>[2x]IVGGRRARPHAWPFMVSLQLRGGHFCGATLIAPNFVMSAAHCVANVNVRAVRVVLGAHNLSRREPTRQVFAVQRIFENGYDPVNLLNDIVILQLNGSATINANVQVAQLPAQGRRLGNGVQCLAMGWGLLGRNRGIASVLQELNVTVVTSLCRRSNVCTLVRGRQAGVCFGDSGSPLVCNGLIHGIASFVRGGCASGLYPDAFAPVAQFVNWIDSIIQ;>[2x]GSTIQIPYTITVNGTSQNILSSLT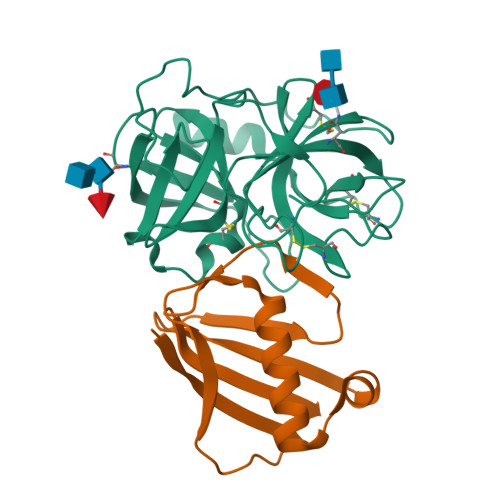FNKNQNISYKDIENKVKSVLYFNRGISDIDLRLSKQAEYTVHFKNGTKRVIDLKSGIYTADLINTSDIKAISVNVD> GYGSWEIDPKDLTFLKELGTGQFGVVKYGKWRGQYDVAIKMIKEGSMSEDEFIEEAKVMMNLSHEKLVQLYGVCTKQRPIFIITEYMANGCLLNYLREMRHRFQTQQLLEMCKDVCEAMEYLESKQFLHRDLAARNCLVNDQGVVKVSDFGLSRYVLDDEYTSSVGSKFPVRWSPPEVLMYSKFSSKSDIWAFGVLMWEIYSLGKMPYERFTNSETAEHIAQGLRLYRPHLASEKVYTIMYSCWHEKADERPTFKILLSNILDV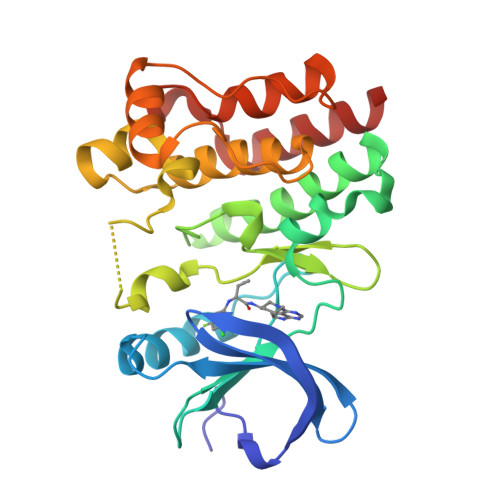MDEES>[3x]GAMAVIDNSTKTLEQQTAQTNVAALPAITVKAEQDDTYAGGQVATSSNVGFLGSKKFLDTPFNTISYTDKYIEDKQAKDITEVIAATDPSIYTNGASGGWSENYYIRGYASSTNDMSMNGLFGITPFYRTSPEMFGRVEVLKGPSALLNGMPPAGSVGGTVNLVTKYAADEPFARLTTTYMSDAQFGGHV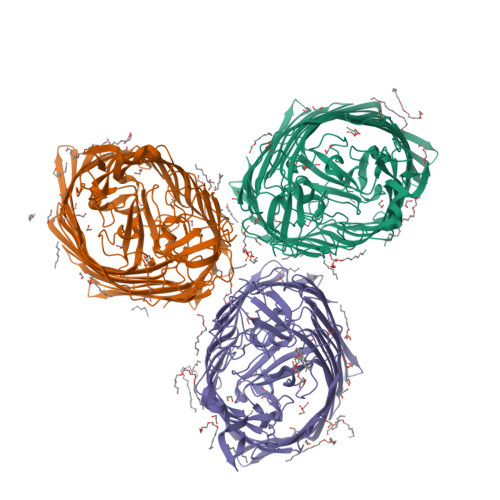DVGRRFGENKEFGVRINGMYRDGDAAVNDQSKESRLFSLGLDWQGENARVFVDAYDALDHVDGVTRGVNVSTAVGIPKPPKADTLLSPDWGSVETKDKGAMIRGEYDFSDQLMAYAAYGQSTTEYKYNGASAGTITSSTGTLSSTLGQLAFDVDKKSADAGFKGKFETGSVKHQWVANATYYNHTQDDYGYRIIPGFSDPVITNIYDPNPNWGPKPEFTPPFLFHSTLSTSSFGLADTLSFAQDKVQLTLGLRHQTVKATSSVNTLPENAKSATTPGVALLIKATDKISVYANYIEGLTKGDQAPATASNPGEIFPPQKTKQQELGLKVDLGTFAHTLSAFEITKPSSYLDPSKLVNNLPTFVSDGEQRNRGIEWSFFGSPIEHVRLMGGFTYLDPELTKTKSGGNDGHTAVAVPKNQAKLGAEWDTQVAQGTLTLSGNINAVSKQYINAENTLSVPGRTLLDVGARYSTKVEDHPVTFRANIYNLTNKAYWAQPQLTNLALGAPRTYMLSVSYDF>MYPSIKETMRVQLSMEGSVNYHAFKCTGKGEGKPYEGTQSLNITITEGGPLPFAFDILSHAFQYGIKVFAKYPKEIPDFFKQSLPGGFSWERVSTYEDGGVLSATQETSLQGDCIICKVKVLGTNFPANGPVMQKKTCGWEPSTETVIPRDGGLLLRDTPALMLADGGHLSCFMETTYKSKKEVKLPELHFHHLRMEKLNISDDWKTVEQHESV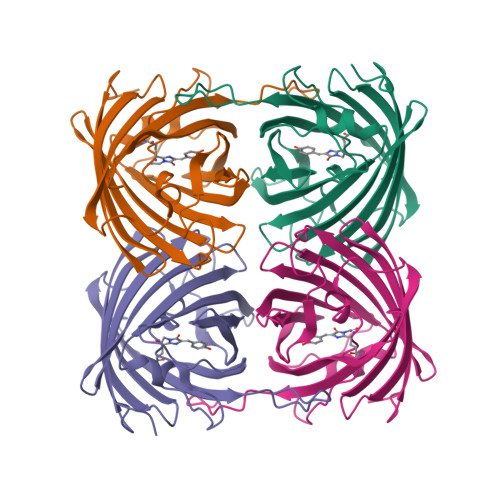VASYSQVPSKLGHN[8x]>[8x]MSFTYKRLDKNDAAVLFVDHQAGLLSLVRDFSPDEFKNNVLALADIARFFNLPTILT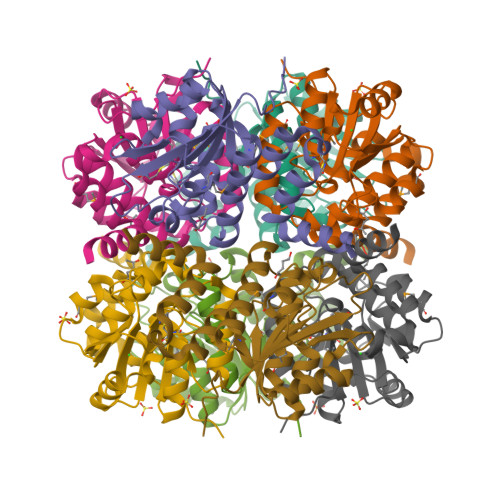TSFEDGPNGPLVPELKEMFPQAPYIARPGNINAWDNEDFVKAVKATGKKQLIIAGVVTDVCVAFPTLSALEEGFDVFVVTDASGTFNPVVRDAAWARMTAAGAQLMNWFSVGCELHRDWRNDIEGFGAILGGHLPAYANLIQSFGTKK His domain protein tyrosine phosphatase (HD-PTP/PTPN23) is a tumor suppressor that regulates mitogenic receptor downregulation, endocytic recycling, and cell migration (Chen et al., 2012, Doyotte et al., 2008, Kharitidi et al., 2015, Lee et al., 2007, Ma et al., 2015, Manteghi et al., 2016). A central feature of HD-PTP function is the ability of its Bro1 domain to recruit CHMP4, the major subunit of the ESCRT-III membrane remodeling protein complex (Doyotte et al., 2008, Ichioka et al., 2007, Parkinson et al., 2015). Crystallographic structures of the HD-PTPBro1 domain in complex with the relevant binding regions of SARA, endofin, and all three human CHMP4 isoforms reveal that SARA and endofin binding is similar to that of CHMP4 at the conserved site, but critically extends into a neighboring specific pocket unique to HD-PTP. Altogether, this study identifies the Bro1 domain of HD-PTP as a highly selective interaction hub that coordinates recruitment of endosomal signaling adaptors versus MVB sorting and receptor degradation.

We also showed that the equivalent region of SARA binds to HD-PTPBro1 (KD 11.3 ± 0.3 μM). As predicted, the 22-mer SARA/endofin peptides form amphipathic α helices in their complexes with HD-PTPBro1. They occupy a larger binding site than the CHMP4 peptides, partially overlapping with the common site across H5, H6, and H7, but extending further into the S site between H3 and H5. The SARA/endofin-HD-PTPBro1 binding interface is largely hydrophobic and involves residues F5, A9/V9, L12, L16, and F19 present in both peptides. SARA/endofin peptides lack the Trp residue conserved in the CHMP4 peptides, but L12 occupies the analogous position, binding to one of the hydrophobic pockets and interacting with L189 in HD-PTPBro1. The smaller size of Leu versus Trp means that fewer rearrangements of this pocket are necessary to accommodate the SARA/endofin versus CHMP4 peptides. Rearrangement mostly consists of a displacement of the R198 side chain and a slight movement of the K141 and K192 side chains. Leu16 accommodates itself into the second hydrophobic pocket and interacts with L202/I206 in the endofin-HD-PTPBro1 complex and I206 in the SARA-HD-PTPBro1 complex, consistent with the importance of these residues for SARA/endofin binding to HD-PTP. Phenylalanine residues (F5 and F19), at both ends of the α helices, anchor SARA/endofin peptides into the binding site. Phe19 forms multiple interactions at the common site, including with L202/I206, while F5 fits into the S site forming several van der Waals contacts.

>MEAVPRMPMIWLDLKEAGDFHFQPAVKKFVLKNYGENPEAYNEELKKLELLRQNAVRVPRDFEGCSVLRKYLGQLHYLQSRVPMGSGQEAAVPVTWTEIFSGKSVAHEDIKYEQACILYNLGALHSMLGAMDKRVSEEGMKVSCTHFQCAAGAFAYLREHFPQAYSVDMSRQILTLNVNLMLGQAQECLLEKSMLDNRKSFLVARISAQVVDYYKEACRALENPDTASLLGRIQKDWKKLVQMKIYYFAAVAHLHMGKQAEEQQKFGERVAYFQSALDKLNEAIKLAKGQPDTVQDALRFTMDVIGGKYNSAKKDNDFIYHEAVPALDTLQPVKGAPLVKPLPVNPTDPAVTGPDIFAKLV[4x];>[2x]MENYFQAEAYNLDKVLDEFEQN(2S)-2-[[4-[[1-[(3,4-dichlorophenyl)methyl]-3,7-dimethyl-2,6-bis(oxidanylidene)purin-8-yl]amino]phenyl]carbonylamino]pentanedioic 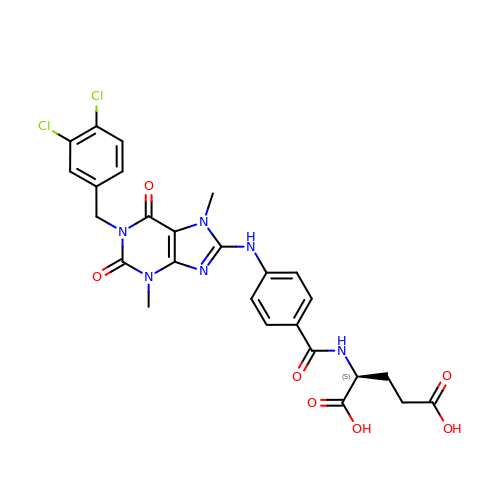acid | C26 H24 Cl2 N6 O7 | VGQGEPKBLLWTIL-SFHVURJKSA-N> APSLNQDIHVQKESEYPAWWKEAVFYQIYPRSFKDTNDDGIGDIRGIIEKLDYLKSLGIDAIWINPHYDSPNTDNGYDISNYRQIMKEYGTMEDFDSLVAEMKKRNMRLMIDVVINHTSDQHPWFIQSKSDKNNPYRDYYFWRDGKD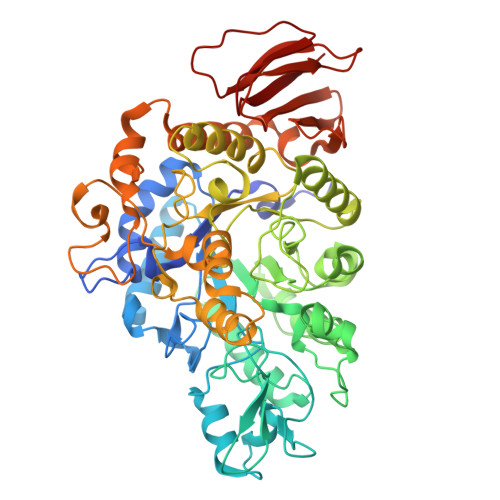NQPPNNYPSFFGGSAWQKDAKSGQYYLHYFARQQPDLNWDNPKVREDLYAMLRFWLDKGVSGMRFDTVATYSKIPGFPNLTPEQQKNFAEQYTMGPNIHRYIQEMNRKVLSRYDVATAGEIFGVPLDRSSQFFDRRRHELNMAFMFDLIRLDRDSNERWRHKSWSLSQFRQIISKMDVTVGKYGWNTFFLDNHDNPRAVSHFGDDRPQWREASAKALATITLTQRATPFIYQGSELGMTNYPFRQLNEFDDIEVKGFWQDYVQSGKVTATEFLDNVRLTSRDNSRTPFQWNDTLNAGFTRGKPWFHINPNYVEINAEREETREDSVLNYYKKMIQLRHHIPALVYGAYQDLNPQDNTVYAYTRTLGNERYLVVVNFKEYPVRYTLPANDAIEEVVIDTQQQAAAPHSTSLSLSPWQAGVYKLR>PAARVEYIAPWWVVWLHSVPHLGLRLQRVDSTFSPGDETYQESLLFLGVLAAIGLGLNLIFLTVYLVCTCCCRRDHTVQTKQQESCCVTWTAVVAGLLCCAAVGVGFYGNSETNDGMHQLIYSLDNANHTFSGMDELVSANTQRMKVDLEQHLARLSEIIAARGDYIQTLKFMQQMAGNVVSQLSGLPVWREVTTQLTKLSHQTAYVEYYRWLSYLLLFILDLVICLVTCLGLARRSKCLLASMLCCGILTLILSWASLAADAAAAVGTSDFCMAPDIYILNNTGSQINSEVTRYYLHCSQSLISPFQQSLTTFQRSLTTMQIQVGGLLQFAVPLFPTAEKDLLGIQLLLNNSEISLHQLTAMLDCRGLHKDYLDALTGICYDGIEGLLFLGLFSLLAALAFSTLTCAGPRAWKYFINRDRDYDDIDDDDPFNPQARRIAAHNPTRGQLHSFCSYSSGLGSQCSLQPPSQTISNAPVSEYMNQAILFGGNPRYENVPLIGRGSPPPTYSPSMRPTYMSVADEHLRHYEFPSSNSLEVLFQ[2x]

Tweety homologs (TTYHs) are conserved transmembrane proteins present in all eukaryotes including three members (TTYH1, TTYH2, and TTYH3) in humans. TTYHs have been reported to form Ca2+- and cell volume-regulated anion channels structurally distinct from any characterized protein family with potential roles in cell adhesion, migration, and developmental signaling. Each protomer consists of five transmembrane helices (TM1–5) and an extracellular domain (ED) which extends 75 Å from the membrane surface between an extracellular N-terminus and intracellular C-terminus. We conclude TTYHs are not pore forming subunits of anion channels and their function may involve Ca2+-dependent changes in quaternary structure, interactions with hydrophobic molecules near the extracellular membrane surface, and/or association with additional protein partners.

Full-length Mus musculus TTYH2 was expressed in HEK293T cells with a cleavable C-terminal fusion to EGFP, extracted and purified in detergent, and reconstituted into lipid nanodiscs formed by the scaffold protein MSP1E3D1 and lipids in the presence of 1 mM Ca2+. We determined the cryo-EM structure of TTYH2 in the presence of Ca2+ to 3.3 Å resolution. The map enabled de novo modeling of 396 of 532 amino acids from each 59 kDa TTYH2 protomer chain with the majority of unmodeled residues within the unstructured C-terminal region (amino acids 415–532) and others within poorly resolved segments of the N-terminus and intracellular loops. In the presence of calcium, TTYH2 adopts a side-by-side homodimer (a “cis-dimer”) within a single nanodisc membrane. Association between TTYH2 protomers in the cis-dimer buries an interface of 1556 Å2 and involves residues in the transmembrane and EDs, primarily in TM2, TM5, EDH1, EDH3d, EDH4a, and EDH4b. A striking feature of the interface is the close juxtaposition of a surface formed by conserved negatively charged or electronegative residues from each protomer in the ED just above the membrane surface. This region includes residues from EDH1 (Y109, S112, E113, and E116) and EDH4b (D384 and E387) with Y109 and S112 underneath E113, E116, D384, and E387. The cryo-EM map contains strong density in the space between the charged residues bridging opposing protomers. Based on electrostatic and geometric features of this site, we speculate that these densities correspond to coordinated Ca2+ ions that would reduce repulsion otherwise expected to occur between the electronegative surfaces of each protomer. In TTYH2 cis-dimers, we observe horseshoe-shaped density within the pocket, although the density is not sufficiently featured at this resolution to unambiguously identify and model.>MHAALSPLSQRFERIAVQPLTGVLGAEITGVDLREPLDDSTWNEILDAFHTYQVIYFPGQAITNEQHIAFSRRFGPVDPVPLLKSIEGYPEVQMIRREANESGRVIGENWHTDSTFLDAPPAAVVMYAKEIPPYGGDTLFTSMYTAWETLSPTMQATIEGLNVVHSATRVFGSLYQAQNRRFSNTSVKVMDVDAGDRETVHPLVVTHPETGRKGLYVNQVYCQRIEGMSEKESEPLLSFLFAHATKPEFTCRVRWQEGDVLVWDNLCTQHYAVPDYAGKFRYLTRTTVGGVRPARHHHHHH[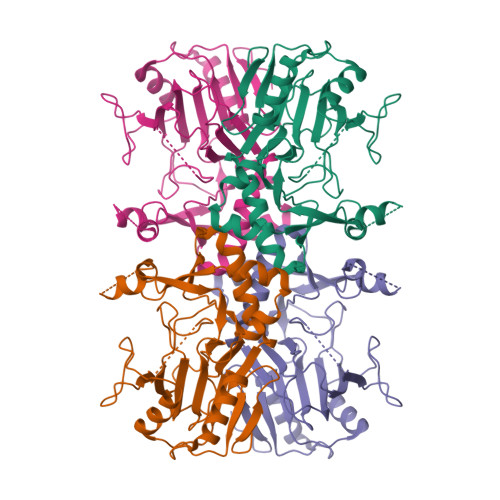8x]> GMSPMTIPSEMKALLLVGDGYTKTPSGSALEAMEPYLEQGRIAVPAPGPSQVLIKVNLASINPSDVAFIKGQYGQPRVKGRPAGFEGVGTIVAGGDEPYAKSLVGKRVAFATGLSNWGSWAEYAVAEAAACIPLLDTVRDEDGAAMIVNPLTAIAMFDIVKQEGEKAFVMTAGASQLCKLIIGLAKEEGFRPIVTVRRDEQIALLKDIGAAHVLNEKAPDFEATLREVMKAEQPRIFLDAVTGPLASA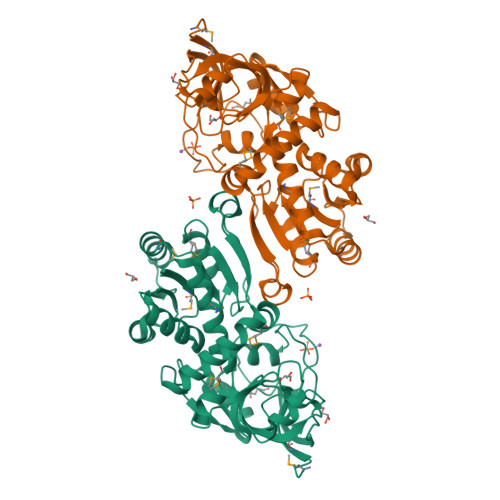IFNAMPKRARWIIYGRLDPDATVIREPGQLIFQHKHIEGFWLSEWMRQFKERRGPAILEAQKRFSDGRWSTDVTAVVPLAEAIAWVPAELTKPNGKVFIRP>[3x]MKHLTTMSELSTEEIKDLLQTAQELKSGKTDNQLTGKFAANLFFEPSTRTRFSFEVAEKKLGMNVLNLDGTSTSVQKG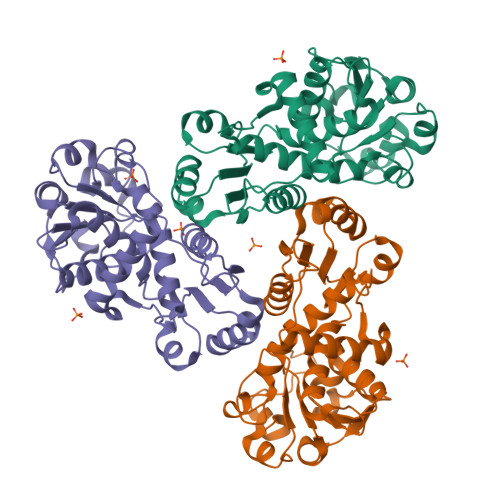ETLYDTIRTLESIGVDVCVIRHSEDEYYEELVSQVNIPILNAGDGCGQHPTQSLLDLMTIYEEFNTFKGLTVSIHGDIKHSRVARSNAEVLTRLGARVLFSGPSEWQDEENTFGTYVSMDEAVESSDVVMLLRIQNERHQSAVSQEGYLNKYGLTVERAERMKRHAIIMHPAPVNRGVEIDDSLVESEKSRIFKQMKNGVFIRMAVIQRALQTNVKRGEAAYVISH>MAAGNAQIGKLAPDFTAKAVMPDGQFKDLKMSDYRGKYVVFFFYPLDFTFVCPTEIIAFSDAADDFKKIGCEVIAASVDSHFSHLAWINTPRKQGGLGTMKIPLVSDTRRTISTDYGVLKEDDGIAYRGLFIIDDKGILRQITIND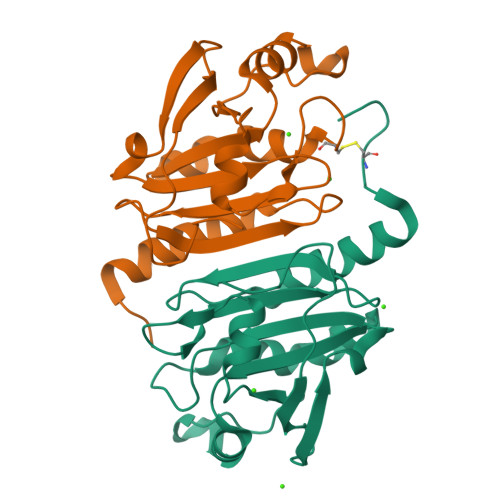LPVGRSVEETLRLVQAFQFTDKHGEVCPAGWKPGSDTIKPDVQKSKDFFSKQ[10x]A conserved family of N-acetylgalactosaminyl-transferases (GalNAc-Ts) initiate mucin-type O-glycosylation by catalyzing GalNAc transfer from uridine 5′-diphosphate (UDP)–GalNAc to a Thr/Ser on a protein to form Thr/Ser–O-GalNAc. GalNAc-Ts are Golgi-anchored type II membrane proteins containing two luminal domains that are important for activity, including an N-terminal Mn2+-dependent catalytic domain that adopts a glycosyltransferase family A (GT-A) fold. The lectin domain consists of three homologous repeats (α, β, and γ), where α and β, but not γ, have GalNAc-binding potential. The isoenzyme GalNAc-T1 is highly expressed in most tissue types and influences many biological pathways, including salivary gland function, heart development, immune system function, and viral infectivity.

To further validate our biochemical data, we attempted to crystallize both human and mouse GalNAc-T1 (98% identity overall, and 99% identity in the lectin domain) with various glycopeptide substrates but were only able to obtain crystals and an x-ray crystal structure of mouse GalNAc-T1 in complex with Muc5AC-13, UDP, and Mn2+ (Muc5AC-13: GTT3PSPVPTTSTT13GalNAcSAP) to 2.3-Å resolution. The asymmetric unit contains a dimer with one GalNAc-T1–Mn2+–UDP–(Muc5AC-13)2 complex (A) having well-resolved electron density and one GalNAc-T1–Mn2+–UDP–(Muc5AC-13)1 complex (B) with poor electron density. The analysis centers on complex A, where GalNAc-T1 is bound to two Muc5AC-13 glycopeptides, one via the α repeat and the other via the β repeat. The Muc5AC-13 glycopeptide interacting with the β repeat GalNAc binding pocket via Thr13–O-GalNAc correctly positions the acceptor Thr3 into the active site for catalysis. However, the 2Fobs-Fcalc electron density for peptide residues beyond Thr10 is not clear and does not provide evidence that the α repeat correctly positions this glycopeptide into the active site for catalysis. Asp444, His460, and Asn465 are involved in hydrogen bonding to GalNAc in the α repeat, while residues Asp484, His498, and Asn503 participate in hydrogen bonds with GalNAc in the β repeat. β repeat GalNAc-T1 residue Lys496 makes hydrogen bonds with peptide residues Thr9 and Thr10 and a backbone carbonyl in β-bound Muc5AC-13. Glu450 in α repeat of GalNAc-T1 interacts with Lys496 in the β repeat and Thr10 in the β-bound Mu5AC-13, suggesting the presence of intra-lectin domain communications. In addition, Glu450 in the α repeat interacts with Lys496 in the β repeat and Thr10 in the β-bound Muc5AC-13. These interactions can mediate communication between the repeats and further support the observations that Thr–O-GalNAc binding in the β repeat could have long-range effects on GalNAc binding in the α repeat and vice versa.

>[2x]MRKFAYCKVVLATSLVWVLLDMFLLLYFSECNKCEEKQERGLPAGDVLELVQKPHEGPGEMGKPVVIPKEDQEKMKEMFKINQFNLMASEMIALNRSLPDVRLEGCKTKVYPDNLPTTSVVIVFHNEAWSTLLRTVHSVINRSPRHMIEEIVLVDDASERDFLKRPLESYVKKLKVPVHVIRMEQRSGLIRARLKGAAVSRGQVITFLDAHCECTAGWLEPLLARIKHDRRTVVCPIIDVISDDTFEYMAGSDMTYGGFNWKLNFRWYPVPQREMDRRKGDRTLPVRTPTMAGGLFSIDRDYFQEIGTYDAGMDIWGGENLEISFRIWQCGGTLEIVTCSHVGHVFRKATPYTFPGGTGQIINKNNRRLAEVWMDEFKNFFYIISPGVTKVDYGDISSRLGLRRKLQCKPFSWYLENIYPDSQIPRHYFSLGEIRNVETNQCLDNMARKENEKVGIFNCHGMGGNQVFSYTANKEIRTDDLCLDVSKLNGPVTMLKCHHLKGNQLWEYDPVKLTLQHVNSNQCLDKATEEDSQVPSIRDCTGSRSQQWLLRNVTLPEIF;>[3x]GTTPSPVPTTSTTSAP Entry of human immunodeficiency virus type 1 (HIV-1) into target cells involves fusion of viral and cellular membranes, a process mediated by the viral surface protein Env (gp160). In the Golgi apparatus, each protomer is cleaved into two subunits that remain noncovalently associated: an N-terminal surface protein (denoted SU or gp120) and a C-terminal transmembrane protein (denoted TM or gp41). Ultimately, the extended state collapses into its most stable form, a trimer-of-hairpins (TOH), in which the C-HR regions pack in an antiparallel manner into hydrophobic grooves on the outside of the N-HR coiled coil. The thermostable core of the gp41 TOH consists of the three-stranded N-HR coiled coil surrounded by three helical C-HR segments.

Propagating HIV-1 (NL4-3 strain) in the presence of fusion inhibitor C37-KYI led to the selection of the escape mutation Q552R. To determine the structural impact of this mutation, we crystallized a construct composed of 40 residues from the N-HR sequence (N40) and 37 residues from the C-HR sequence (C37) and solved its structure. Although the mutant six-helix bundle crystallized in a hexagonal space group (P31), three-fold crystallographic symmetry did not run through the center of the N-HR coiled coil as it does in almost all previous gp41 TOH structures. Instead, the structure was markedly asymmetric in that only two of the three N40 segments were folded into α-helices throughout their entire length. The N-terminal region (residues 545–554) of the third N40 segment assumed a distorted, largely extended conformation. However, by residue 555 (three residues C-terminal to the Q552R mutation), this N40 segment resumed a helical fold, restoring three-fold symmetry to the coiled coil. As a consequence of the asymmetric distortion of the N-HR coiled coil, the three Arg552 residues occupied distinctly different chemical environments. One Arg552 side chain extended from an intact N-HR helix into the coiled-coil interior, where it formed a hydrogen bond with the backbone of the other intact N-HR helix. The Arg552 side chain from the second intact N-HR helix reached into an N40/C37 interface, replacing the Gln551 side chain from an adjacent N-HR segment. Thus, in contrast to the wild type N-HR coiled coil, the Q552R-mutant coiled coil possessed dissimilar C37 binding sites, with the distorted N-HR segment substantially disrupting two out of the three sites.

>MQLLSGIVQQRNNMLRAIEAQQHLLQLTVWGIKQLQARILAGGRGGHTTWMEWDREINNYTSLIHSLIEESQNQQEKNEQELLGGHHHHHH[3x]>[24x]MAYRFIKWFEELSKNDVPLVGGKGANLGEMTNAGIPVPPGFCV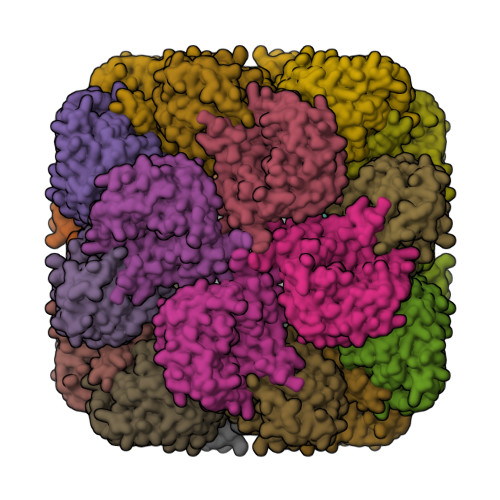TAEAYKYFVENVKVSKEDVKRILGEKVNKGTISEVLAQAPDEPRPLQDWIMDIISKTDVDDSKMLQENTEAIRTLIKSLDMPSEIAEEIKQAYKELSQRFGQEEVYVAVRSSATAEDLPEASFAGQQETYLDVLGADDVIDKVKRCWASLWTARATFYRAKQGFDHSKVYLSAVVQKMVNSEKSGVMFTANPVTNNRNEIMINASWGLGEAVVSGAVTPDEYIVEKGTWKIKEKVIAKKEVMVIRNPETGRGTVMVKVAEYLGPEWVEKQVLTDEQIIEVAKMGQKIEDHYGWPQDIEWAYDKDDGKLYIVQSRPITTLKEEATAEEAEEVEEAEVILKGLGASPGIGAGRVVVIFDASEIDKVKEGDILVTTMTNPDMVPAMKRAAAIVTDEGGRTSHAAIVSRELGIPCVVGTKEATKKLKTGMYVTVDGTRGLVYKGIVKSLVKKKEEAKAEGGQVVVAGAPLVTGTMVKVNVSMPEVAERAAATGADGVGLLRAEHMILSIGQHPIKFIKEGKEEELVEKLAEGIEKVAAAFYPRPVWYRTLDAPTNEFREMPGGEDEPEERNPMLGWRGIRRGLDQPELLRAEFKAIKKVVEKGYNNIGVMLPLVSHPEQIREAKRIAREVGLEPHKDVAWGVMIEVPAAAIIIEDLIKEGIDFVSFGTNDLTQYTLAIDRDNERVAKLYDETHPAVLKLIKHVIKVCKRYGVETSICGQAGSDPKMARILVRLGIDSISANPDAVQLIRQVVAQEERKLMLEAARKQLFEEEEEEELF> XDE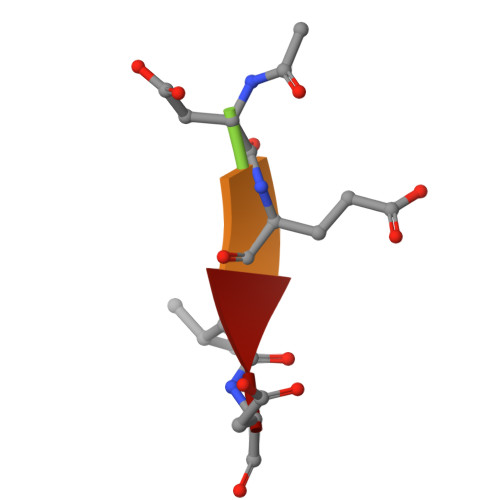VD7-THIONICOTINAMIDE-ADENINE-DINUCLEOTIDE PHOSPHATE | C21 H28 N7 O16 P3 S | 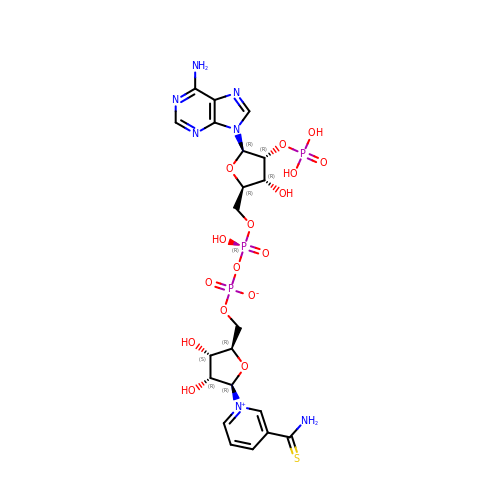OJNFDOAQUXJWED-NNYOXOHSSA-N> GSSSTHAPSSKTLADNIETADLSASVPTRPAEPERKTLADYGGYPSALDAVKQKNDAAVAAYLENAGDSAMAENVRNEWLKSLGARRQWTLFAQEYAKLEPAGRAQEVECYADSSRNDYTRAAELVKNTGKLPSGCTKLLEQAAASGLLDGNDAWRRVRGLLAGRQTTDARNLAAALGSPFDGGTQGSREYALLNVIGKEARKSPNAAALLS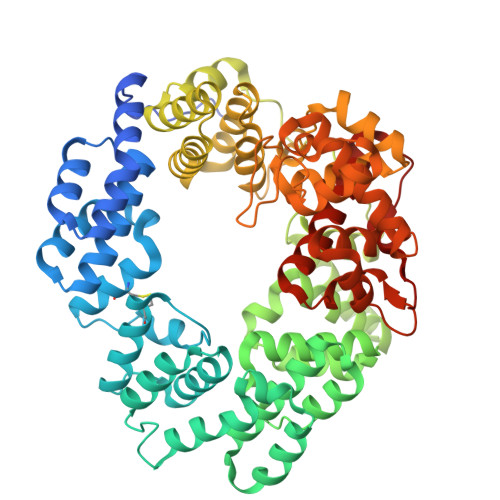EMESGLSLEQRSFAWGVLGHYQSQNLNVPAALDYYGKVADRRQLTDDQIEWYARAALRARRWDELASVISHMPEKLQKSPTWLYWLARSRAATGNTQEAEKLYKQAAATGRNFYAVLAGEELGRKIDTRNNVPDAGKNSVRRMAEDGAVKRALVLFQNSQSAGDAKMRRQAQAEWRFATRGFDEDKLLTAAQTAFDHGFYDMAVNSAERTDRKLNYTLRYISPFKDTVIRHAQNVNVDPAWVYGLIRQESRFVIGAQSRVGAQGLMQVMPATAREIAGKIGMDAAQLYTADGNIRMGTWYMADTKRRLQNNEVLATAGYNAGPGRARRWQADTPLEGAVYAETIPFSETRDYVKKVMANAAYYAALFGAPHIPLKQRMGIVPAR>[2x]GPLGSDYIIKEKTVLLQKKDSEGFGFVLRGAKAQTPIEEFTPTPAFPALQYLESVDEGGVAWRAGLRMGDFLIEVNGQNVVKVGHRQVVNMIRQGGNTLMVKVVMVTRHPDM;>XEAQTRF[2x]

We demonstrate the power of the approach using two unrelated exemplar PPI targets: (i) p53/hDM2, an α-helix-mediated PPI37 that is a clinically relevant oncology target;38 and (ii) GKAP/SHANK1-PDZ,39 a β-strand-mediated PPI which plays a key role at the synaptic junction and is representative of PDZ-mediated interactions, which remain challenging for small-molecule inhibitor discovery. As a β-strand mediated PPI, the GKAP/SHANK1 interface relies on both side-chain contacts and an extensive hydrogen bond network that plays an active role in molecular recognition (H-bonds are shown as orange dashed lines); these features are not readily reproduced by typical (often hydrophobic) small molecule scaffolds. In our prior studies, computational modelling using BudeAlaScan55,56 and experimental analyses confirmed the Thr and Leu amino acids together with the terminal carboxylic acid as crucial for binding. Although SHANK1 has a defined hydrophobic cavity in which the Leu side chain of GKAP is accommodated (magenta area), it represents a significantly more challenging target for small-molecule mimicry than p53/hDM2.

Thus, for query generation, the key hot residues of GKAP together with backbone heteroatoms were used. However, when our workflow was implemented with a query bearing these features, we identified only flexible peptide-based inhibitor candidates (not shown). We reasoned that the C-terminal leucine, with more side-chain degrees of freedom, might have contributed to the moderate results in our in silico structure similarity analyses. The plasticity of PDZ domains allows the accommodation of various hydrophobic side chains at the C-terminus of the peptide; for SHANK1, Leu dominates for C-terminal carboxylates, however Phe has been observed to dominate for non-C-terminal sequences. Therefore, we considered Phe, with its more rigid hydrophobic amino acid sidechain, as a suitable surrogate in this position of the query. Gratifyingly, preparation of the Ac-Glu-Ala-Gln-Thr-Arg-Phe-CO2H peptide and assessment by isothermal titration calorimetry confirmed the Phe variant peptide to be tolerated (Kd = 5 (±0.5) μM compared with Kd = 2 (±0.3) μM for the GKAP sequence) and to act as an effective inhibitor (Fig. 3f and S11† for fluorescence competition anisotropy assay data using FAM-Ahx-Glu-Ala-Gln-Thr-Arg-Leu-CO2H as tracer). Application of the in silico screening workflow to a modified query with the Phe substitution identified a number of small-molecule candidate inhibitors (i and S12†). These candidates were screened in a fluorescence anisotropy competition assay at 30 and 300 μM following a similar approach to that pursued for the p53/hDM2 interaction, although a smaller number of less potent hits were obtained. Compound Z-1 had an IC50 ∼ 300 μM in a fluorescence anisotropy competition assay.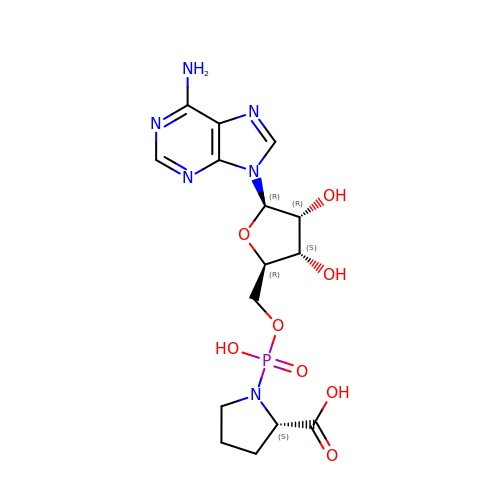(2~{S})-1-[[(2~{R},3~{S},4~{R},5~{R})-5-(6-aminopurin-9-yl)-3,4-bis(oxidanyl)oxolan-2-yl]methoxy-oxidanyl-phosphoryl]pyrrolidine-2-carboxylic acid | C15 H21 N6 O8 P | YHPWCYBNNLQQNG-TWBCTODHSA-N> MAEEHHHHHHHHLEVLFQGPPPGPRSPQREPQRVSHEQFRAALQLVVDPGDPRSYLDNFIKIGEGSTGIVCIATVRSSGKLVAVKKMDLRKQQRRELLFNEVVIMRDYQHENVVEMYNSYLVGDELWVVMEFLEGGALTDIVTHTRMNEEQIAAVCLAVLQALSVLHAQGVIHRDIKSDSILLTHDGRVKLSDFGFCAQVSKEVPRRKSLVGTPYWMAPELISRLPYGPEVDIWSLGIMVIEMVDGEPPYFNEPPLKAMKMIRDNLPPRLKNLHKVSPSLKGFLDRLLVRDPAQRATAAELLKHPFLAKAGPPASIVPLMRQNRTR;> AEDWTAALLNRGRSRQPLVLGDNC

PAK4 is a kinase with strong links to cellular transformation and cancer metastasis, as reviewed. We have shown that Cdc42 directly regulates PAK4 activity in mammalian cells through an auto-inhibitory domain (AID) that binds in a manner similar to pseudosubstrates. We have identified Inka1 as a potent vertebrate inhibitor of PAK4 with a Ki of ∼30 nM, which has a much higher affinity than the corresponding AID. The recombinant 38 amino acid ‘Inka box' (GST-iBox) is a potent of PAK4cat inhibitor in vitro but does not affect PAK1, suggesting Inka1 is a specific group II PAK30 inhibitor.

On the basis of these experiments, we hypothesize that Inka1 stabilizes the ATP-bound crystallization-competent conformation of the kinase domain by preventing ATP hydrolysis through binding tightly in the cleft between the N- and C-lobes. This in-cellulo iBox–PAK4cat structure determined in space group P63 was verified by comparison with the structure of the complex determined at 2.0 Å resolution from P41212 crystals grown in vitro from purified PAK4cat and a synthetic iBox 24mer peptide. The packing between the N-lobes, as observed in the in-cellulo P63 crystal form, is also reproduced in the in-vitro P41212 crystal reported here and elsewhere121431424344, and in an in-vitro P212121 crystal, demonstrating that this interaction is conducive for crystallization. These two crystal forms support a range of apo peptide inhibitors and small-molecule inhibitor complexes with PAK4cat. The disposition of the core Inka1 sequence (RSRQPLVLGD) in the current structure shows docking in to the substrate-binding pocket (primarily via R-2 and R-4 interactions) and the inhibitor chain runs parallel to, and hydrogen bonds with, several main-chain residues of the activation loop in a β-sheet-like manner. The AID and Inka1 structures similarly feature Arg-mediated salt bridges that bind an acidic pocket and hydrophobic side-chain interactions at the +2 and +3 positions.> MARTGAEYIEALKTRPPNLWYKGEKVEDPTTHPVFRGIVRTMAALYDLQHDPRYREVLTYEEEGKRHGMSFLIPKTKEDLKRRGQAYKLWADQNLGMMGRSPDYLNAVVMAYAASADYFGEFAENVRNYYRYLRDQDLATTHALTNPQVNRARPPSGQPDPYI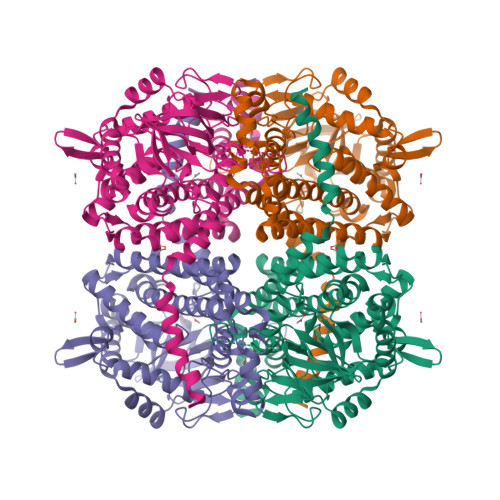PVGVVKQTEKGIVVRGARMTATFPLADEVLIFPSILLQAGSEKYALAFALPTSTPGLHFVCREALVGGDSPFDHPLSSRVEEMDCLVIFDDVLVPWERVFILGNVELCNNAYGATGALNHMAHQVVALKTAKTEAFLGVAALMAEGIGADVYGHVQEKIAEIIVYLEAMRAFWTRAEEEAKENAYGLLVPDRGALDGARNLYPRLYPRIREILEQIGASGLITLPSEKDFKGPLGPFLEKFLQGAALEAKERVALFRLAWDMTLSGFGARQELYERFFFGDPVRMYQTLYNVYNKEPYKERIHAFLKESLKVFEEVQA(2R)-3-{[(S)-(2-aminoethoxy)(hydroxy)phosphoryl]oxy}-2-(tetradecanoyloxy)propyl 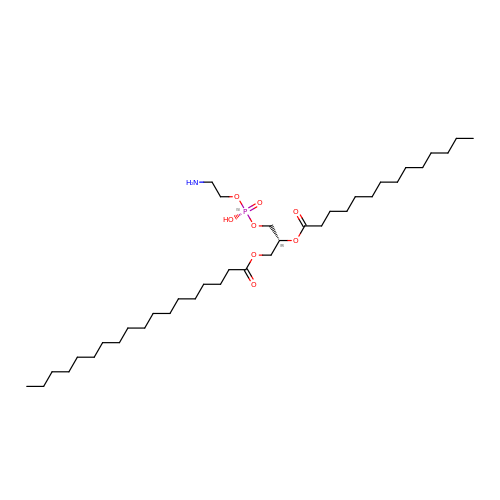octadecanoate | C37 H74 N O8 P | RFJQNULIDFTTLL-PGUFJCEWSA-N>[3x]PAIQSELDVNGEDFARNREAMLAAVAGFRELEQKVLDKAAEARPKFEKRGQLLPRERLALLLDPGAPFLELSSLAGYKLHDDKDGTQAGGGIIAGIGYIAGVRCLVSASNSAIKGGTISPTGLKKTLRLQQIAMENKLPVVTLTESGGANLNYAAEIFVEGARGFANQARISAMGIPQVTVVHGSSTAGGAYQPGLSDYVVVVRGKAKMFLAGPPLLKAATGEIASDEELGGAELHAQVAGTAEYLAENDADGVRLAREIVGMLPWNAQLPARPARSWREPLYPVEELLGVVPADPKKPYDVREIVARIADGSEFLDFKNEFDGQTVCGHLRIEGHACGLIGNNGPITPQGAAKAAQFIQLCEQSNTPLLFLHNTTGFMVGTESERQGVIKHGSKMIQAVANARVPKLTLVVGGSYGAGNYAMCGRGLDPRFIFAWPNSRTAVMGGAQAGKVLRIVTEEKHAKEGKEADPKMLEMLETVTAQKLDSQSTALYGTASLWDDGLVDPRDSRRLLGYLLDICAEAEARPLKGNSFGVARF

Geranyl-CoA carboxylase (GCC) activity was first purified from a Pseudomonas organism grown with either the related acyclic monoterpenoid citronellol or geranic acid as the sole carbon source. GCC also possesses 3-methylcrotonyl-CoA carboxylase (MCC) activity, and 3-methylcrotonyl-CoA is an intermediate in the complete catabolism of citronellol and geranic acid. GCC and MCC are members of the biotin-dependent carboxylase superfamily. Both consist of two subunits, α and β, and their holoenzymes are 750-kDa-α6β6 dodecamers.

We first determined the structure of Pseudomonas aeruginosa GCC (PaGCC) β subunit at 2.4 Å resolution. The structure confirms our hypothesis, showing that GCCβ has the same connectivity between its N and C domains as that of MCCβ. The overall structures of the two subunits are similar, with root mean squared distance of 1.2 Å for 464 equivalent Cα atoms between them, consistent with their strong sequence conservation. The overall structures of the two β6 hexamers are similar to each other as well, with root mean squared distance of 1.3 Å for 2,866 equivalent Cα atoms. While the connectivity in GCCβ is the same as in MCCβ, the linker between the N and C domains has a different conformation. In addition, the C-terminal segment of GCCβ (residues 526–538) contacts the N domain, while that of MCCβ contacts the C domain. The long helix at the N-terminal end of GCCβ is disordered in one of the three β subunits in the asymmetric unit, although this helix is fully ordered in the GCC holoenzyme structure. There is a large, mostly hydrophobic pocket at the bottom of the active site in GCC that can accommodate the larger geranyl group. Interestingly, the side chain of Phe191 in MCCβ is located in this pocket and clashes with the second isopentenyl group of geranyl-CoA. The equivalent residue in GCC is Gly162.>[2x]SNALEDSSTISFITWNIDGLDGCNLPERARGVCSCLALYSPDVVFLQEVIPPYCAYLKKRAASYTIITGNEEGYFTAILLKKGRVKFKSQEIIPFPNTKMMRNLLCVNVSLGGNEFCLMTSHLESTRGHSAERIRQLKTVLGKMQEAPDS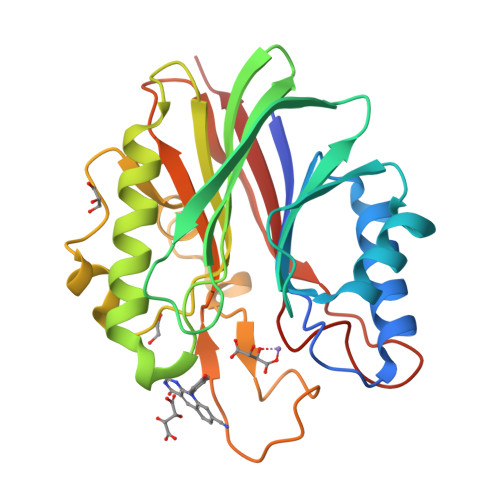TTVIFAGDTNLRDREVIKCGGLPDNVFDAWEFLGKPKHCQYTWDTKANNNLRIPAACKLRFDRIFFRAEEGHLIPQSLDLVGLEKLDCGRFPSDHWGLLCTLNVVL> MYWMNVVIGKMNAEVGGEVVVPIEFNNVPSFGINNCDFKLVYDATALELKNVEAGDIIKTPLANFSNNKSEE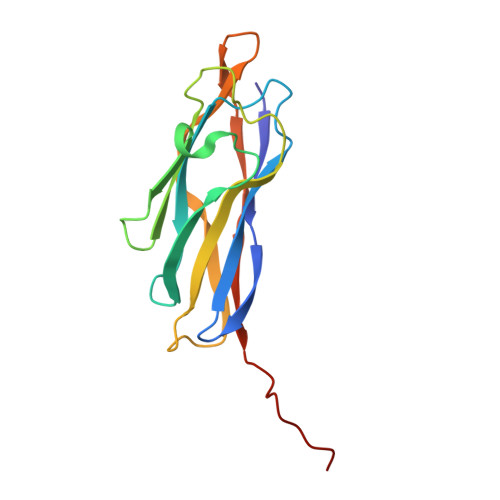GKISFLFNDASQGSMQIENGGVFAKITFKVKSTTATGVYDLRKDLVGSFSGLKDNKMTSIGAEFTNGSITVAATAPLEHHHHHH>AYESIQVTSAQKHVLHVQLNRPEKRNAMNRAFWRELVECFQKISKDSDCRAVVVSGAGKMFTSGIDLMD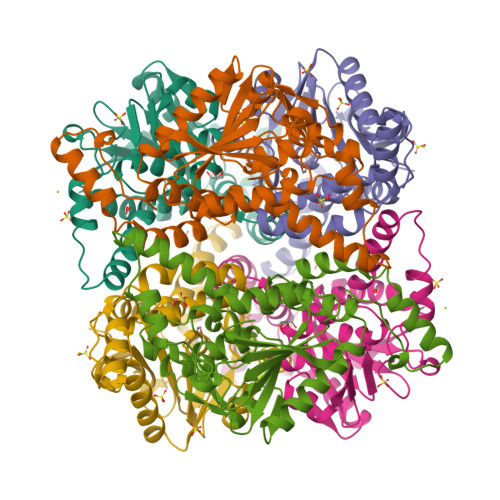MASDILQPPGDDVARIAWYLRDLISRYQKTFTVIEKCPKPVIAAIHGGCIGGGVDLISACDIRYCTQDAFFQVKEVDVGLAADVGTLQRLPKVIGNRSLVNELTFTARKMMADEALDSGLVSRVFPDKDVMLNAAFALAADISSKSPVAVQGSKINLIYSRDHSVDESLDYMATWNMSMLQTQDIIKSVQAAMEKKDSKSITFSKL[3x]Here, we show that a generic and kinetically biased ‘Gembody’ (Gb) interface, previously discovered through trapping in crystallo, can also be trapped in solution by kinetically controlled side-chain-to-side-chain bond formation in a manner that leads to ready generation of complexes; these display ideally balanced interface flexibility and yet relative complex constraints, in turn allowing rapid cryo-EM structure determination, even of small targets. Ultimately, after a survey of in-solution covalent bond-forming methods exploring differing natural and unnatural amino acid residues, we found that Cu(II)-catalyzed oxidation at a pivotal C12 residue site (together with the presence of needed Gb ‘gem’ substitutions previously discovered through iterative X-ray-guided engineering) offered a route to direct and rapid, high-yielding formation of disulfide-linked homo Di-Gembody (homoDiGb) without side reactions (for example, off-site oxidation) to form a robust covalent interface. Furthermore, the success of DiGbs for high-resolution structural solution is enabled by their relatively small mass contribution to the imaged complex while increasing the maximum particle diameter for better particle alignment. In summary, our plug-and-play DiGb strategy improves cryo-EM resolvability and resolution of small proteins through constraint and increased particle size with a simple and robust workflow and can even enable simultaneous structure determination of two challenging targets in one dataset.

To probe the applicability and value of these homoDiGbs to cryo-EM structure determination, we tested the 49-kDa DNA helicase RECQL5 as a challenging soluble target with both small size and substantial interdomain flexibility. Next, a larger dataset of this RECQL5:homoDiGb complex on a 300-kV microscope with standard operating parameters yielded a 3.79-Å reconstruction of the complex after imposing C2 symmetry. Because of minor flexibility within the DiGb interface, imposition of strict C2 symmetry prevents refinement to high-resolution signals. Therefore, we applied an approximate ‘non-strict C2 symmetry’ that improved the alignment of the particle images. In this way, this initial map could be further improved by forgoing strict C2 symmetry, with symmetry expansion and local refinement of RECQL5 alone improving the resolution to 3.18 Å. Current cryo-EM structure determination methods typically struggle with targets below 50 kDa, contrasting with our ready solution of the structure of 49 kDa RECQL5. Further validating these methods, all of the structures obtained were largely consistent with deposited structures, with the only changes being small interdomain movements observed in RECQL5 and its slightly different Gb conformations.

> PERRVRSTLKKVFGFDSFKTPLQESATMAVVKGNKDVFVCMPTGAGKSLCYQLPALLAKGITIVVSPLIALIQDQVDHLLTLKVRVSSLNSKLSAQERKELLADLEREKPQTKILYITPEMAASSSFQPTLNSLVSRHLLSYLVVDEAHCVSQWGHDFRPDYLRLGALRSRLGHAPCVALTATATPQVQEDVFAALHLKKPVAIFKTPCFRANLFYDVQFKELISDPYGNLKDFCLKALGQEADKGLSGCGIVYCRTREACEQLAIELSCRGVNAKAYHAGLKASERTLVQNDWMEEKVPVIVATISFGMGVDKANVRFVAHWNIAKSMAGYYQESGRAGRDGKPSWCRLYYSRNDRDQVSFLIRKEVAKLQEKRGNKASDKATIMAFDALVTFCEELGCRHAAIAKYFGDALPACAKGCDHCQNPTAVRRRLEALERSSSW> KVERKPPDADGCLHADPDLGVLCPTGCKLQDTLVRQERPIRKSIEDLRNTVDSVSRTSSSTFQYITLLKNMWKGRQNQVQDNENVVNEYSSHLEKHQLYIDETVKNNIPTKLRVLRSILENLRSKIQKLESDVSTQMEYCRTPCTVTCNIPVVSGKECEKIIRNEGETSEMYLIQPEDSSKPYRVYCDMKTEKGGWTVIQNRQDGSVDFGRKWDPYKQGFGNIATNAEGKKYCG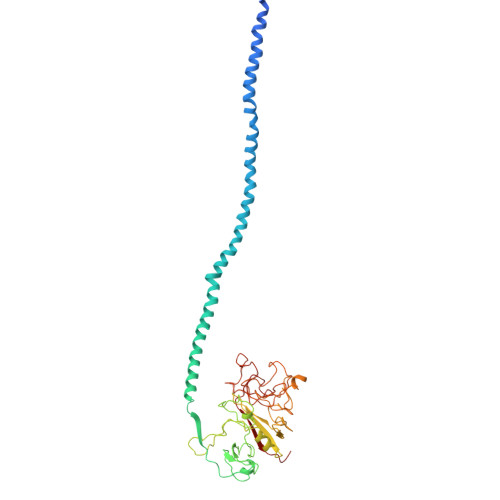VPGEYWLGNDRISQLTNMGPTKLLIEMEDWKGDKVTALYEGFTVQNEANKYQLSVSKYKGTAGNALIEGASQLVGENRTMTIHNSMFFSTYDRDNDGWKTTDPRKQCSKEDGGGWWYNRCHAANPNGRYYWGGAYTWDMAKHGTDDGVVWMNWQGSWYSMKKMSKMIRPYFPEQ>[2x]MEFTYSYLFRMISHEMKQKADQKLEQFDITNEQGHTLGYLYAHQQDGLTQNDIAKALQRTGPTVSNLLRNLERKKLIYRY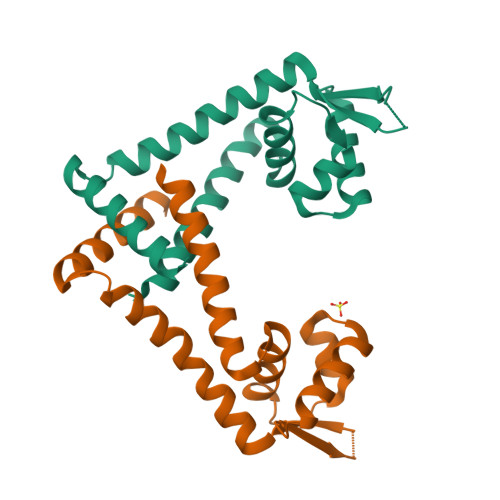VDAQDTRRKNIGLTTSGIKLVEAFTSIFDEMEQTLVSQLSEEENEQMKANLTKMLSSLQ>MLMSVFHNWLLEIACENYFVYIKRLSANDTGATGGHQVGLYIPSGIVEKLFPSINHTRELNPSVFLTAHVSSHDCPDSEARAIYYNSAHFGKTRNEKRITRWGRGSPLQDPENTGALTLLAFKLDEQGGDCKEVNIWVCASTDEEDVIETAIGEVIPGALISGPAGQILGGLSLQQAPVNHKYILPEDWHLRFPSG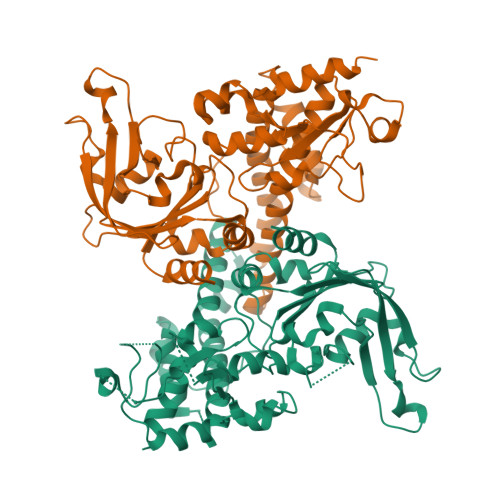SEIIQYAASHYVKNSLDPDEQLLDRRRVEYDIFLLVEELHVLDIIRKGFGSVDEFIALANSVSNRRKSRAGKSLELHLEHLFIEHGLRHFATQAITEGNKKPDFLFPSAGAYHDTEFPVENLRMLAVKTTCKDRWRQILNEADKIHQVHLFTLQEGVSLAQYREMRESGVRLVVPSSLHKKYPEAVRAELMTLGAFIAELTGLYADIP[2x]> APPLVNLAEEKDVKVTVGENMDLKNADLLTDGDKYYLQHDATGNKEGNNWENYQEQGTEVTSTAEGKNGVWVQVDLGASYPLEVINLKRQVYDGQATIGNGNPSGQGKRLKGTKISYKNTAIVIGNEEDLSDGQIVYYEGNPTLPDGVKQPENVSKPYEEAMGGQWFYMDYANKNGLGATELGTTKEARYIRVYTENPKGAAVKFMELGIYGYENEQDVQSQDGPRRVIDNEHPMMIATAYSNDVYEIGQEEGPELQGSNTVDGRWNAIPDDLKENNVLLLHTNNLRQFAPDHIGQAYLQAFHEHGLQIAYEQGAPIMLLGLTAAATPENGGTQYNITADMDYGWLDLMYRMYPNMQGVFNTANFWAGIHPPCEGSAKMLEIADRFGGFFVWSDQDHGSTVTNIVSNANMKKALEKHGDAFYLIYKNTSSNQPDDLKTSSFFQGSWLAGYTGGWGMLSDTWAWDKQFSKLWQGAGSYNNWQRLCGEPEALLGMQMMSTYLGGGVIYTFEFPEIVYGTSNTNSPANTHVLTELFRYIVNHPAPSKKEIMEETKAVLYGNVSSDFYSGLSGKPTGFQIYETGRYGIIPVIPTWGTRAEVTKKLIQEADKLGVTPPNVLDVKDKNLSGQAKQKYFKDLYPIEYVGNAFADKWEGTWYLYNNKVNTNEKQHAILPLEGEEESARLKVEMEPHEFMIM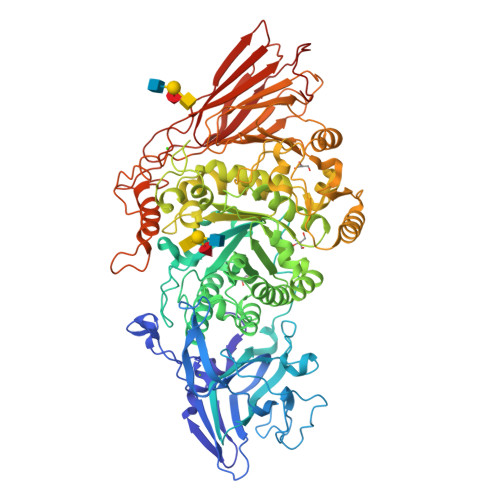NESGDGTAMDITLNNYRVNKDEIIFDNKFGLTWTGDFSPGQTTINGKLSVYKYMDEYNVVNAPEGKLSPEDNELRTTTFELTKLAKEPKVQVVKGQQPDTDGQPQYTEPKVEFNEETGKAVITIQTNGWVDLSITGLEFVYDENAQKIEDE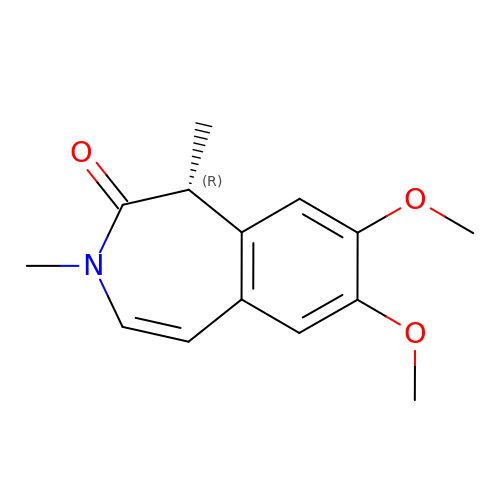(1~{R})-7,8-dimethoxy-1,3-dimethyl-1~{H}-3-benzazepin-2-one | C14 H17 N O3 | DIOZLEANHAFFJH-SECBINFHSA-N> YV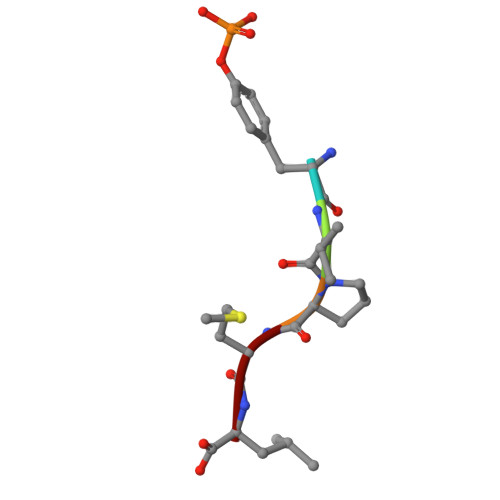PML> MARIRHVQGDITEFQGDAIVNAANNYLKLGAGVAGAILRKGGPSIQEECDRIGKIRVGEAAVTGAGNLPVRYVIHAAVLGDEPASLETVRKATKSALEKAVELGLKTVAFTSWGAWVGGLPAEAVHRVMFEEIKKAPDTLEVTGVHGTEKSAEAYRRALLEHHHHH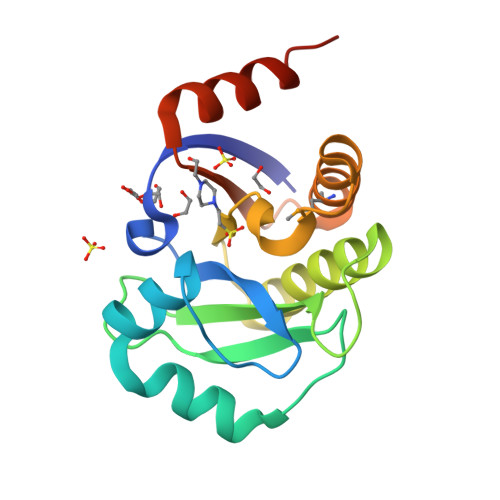H> MALFNTAHGGNIREPATVLGISPDQLLDFSANINPLGMPVSVKRALIDNLDCIERYPDADYFHLHQALARHHQVPASWILAG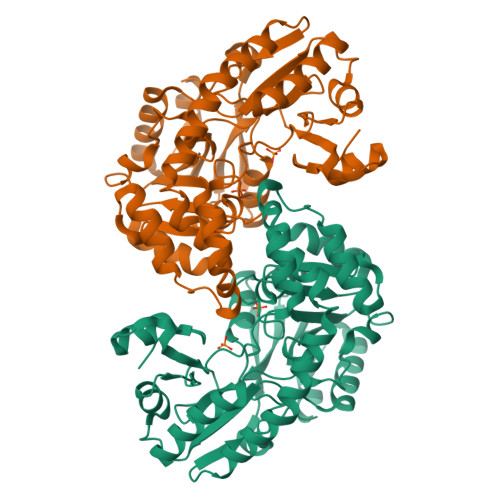NGETESIFTVASGLKPRRAMIVTPGFAEYGRALAQSGCEIRRWSLREADGWQLTDAILEALTPDLDCLFLCTPNNPTGLLPERPLLQAIADRCKSLNINLILDEAFIDFIPHETGFIPALKDNPHIWVLRSLTKFYAIPGLRLGYLVNSDDAAMARMRRQQMPWSVNALAALAGEVALQDSAWQQATWHWLREEGARFYQALCQLPLLTVYPGRANYLLLRCEREDIDLQRRLLTQRILIRSCANYPGLDSRYYRVAIRSAAQNERLLAALRNVLTGIAPAD(5R)-5-methyl-N-[(3S)-5-methyl-4-oxo-2,3,4,5-tetrahydro-1,5-benzoxazepin-3-yl]-4,5,6,7-tetrahydro-2H-indazole-3-carboxamide | C19 H22 N4 O3 | 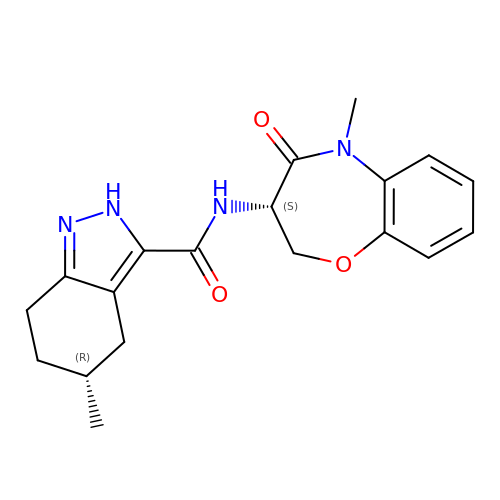LOTYATKNTZKNHI-RISCZKNCSA-N> GHHHHHHHHHHSGENLYFQGHMATFISVQLKKTSEVDLAKPLVKFIQQTYPSGGEEQAQYCRAAEELSKLRRAAVGRPLDKHEGALETLLRYYDQICSIEPKFPFSENQICLTFTWKDAFDKGSLFGGSVKLALASLGYEKSCVLFNCAALASQIAAEQNLDNDEGLKIAAKHYQFASGAFLHIKETVLSALSREPTVDISPDTVGTLSLIMLAQAQEVFFLKATR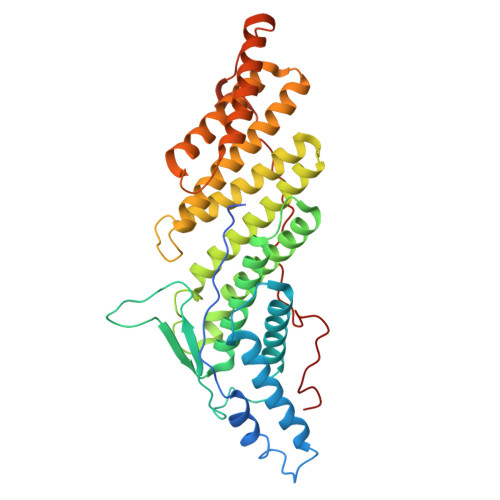DKMKDAIIAKLANQAADYFGDAFKQCQYKDTLPKEVFPVLAAKHCIMQANAEYHQSILAKQQKKFGEEIARLQHAAELIKTVASRYDEYVNVKDFSDKINRALAAAKKDNDFIYHDRVPDLKDLDPIGKATLVKSTPVNVPISQKFTDLFEKMV> MQFPQLDPATLAAFSAAFRGELIWPSDADYDEARRIWNGTIDRRPALIARCTSTPD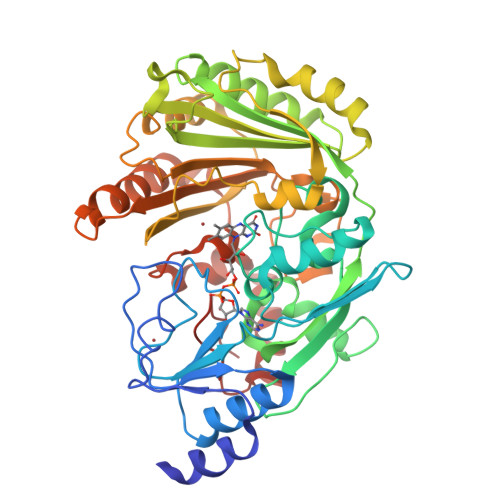VVAAVSFARKSGLLVAVRGGGHSMAGHSVCDGGIVIDLSLMNSIKVSRRLRRARAQGGCLLGAFDTATQAHMLATPAGVVSHTGLGGLVLGGGFGWLSRKYGLSIDNLTSVEIVTADGGVLTASDTENPDLFWAVRGGGGNFGVVTAFEFDLHRVGPVRFASTYYSLDEGPQVIRAWRDHMATAPDELTWALYLRLAPPLPELPADMHGKPVICAMSCWIGDPHEGERQLESILHAGKPHGLTKATLPYRALQAYSFPGAVVPDRIYTKSGYLNELSDEATDTVLEHAADIASPFTQLELLYLGGAVARVPDDATAYPNRQSPFVTNLAAAWMDPTEDARHTAWAREGYRALAGHLSGGYVNFMNPGEADRTREAYGAAKFERLQGVKAKYDPTNLFRLNQNIPPSSP> STGEAIQKLRETENMLIKKQEFLEAKIEDELNIARKNASKNKRVALQALKKKKRLEKQLQQIDGTLSTIEMQREALESANTNT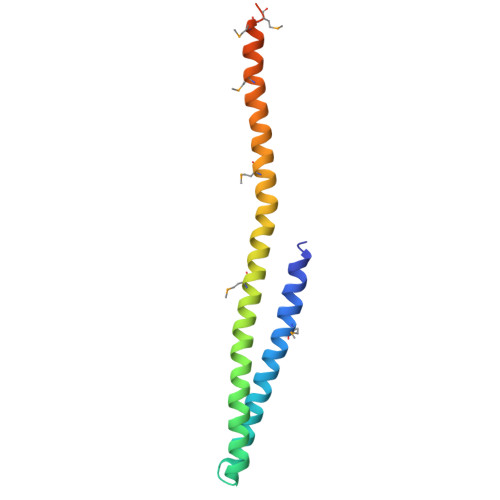AVLTTMKNAADALKRAHQNMDVDKVHDMMDDIAEQQDVAREISD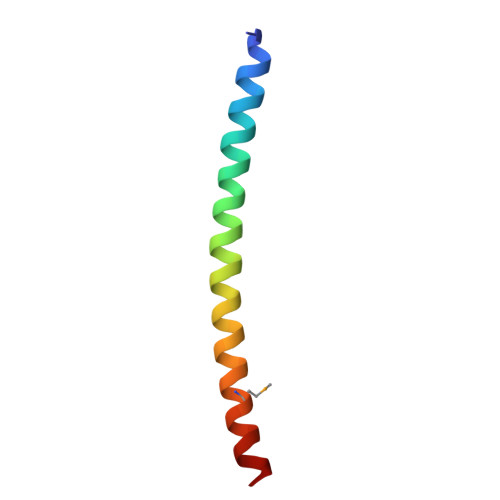> TQQEIFDKQRRLQELSEKVRTCHQEISALRKALQEKEAEMLQVLEDIQT>NLSDVDLSKYITTIAGVMTLSQVKGFVRKNGVNEAKIDEIKNDNVQDTAEQKVQLLRNWHQLHGKKEAYDTLIKDLKKANLCTLAEKIQTIILKDITSDSENSNFRNEIQSLVLE[8x];>[8x]GEEDLCAAFNVICDNVGKDWRRLARQLKVSDTKIDSIEDRYPRNLTERVRESLRIWKN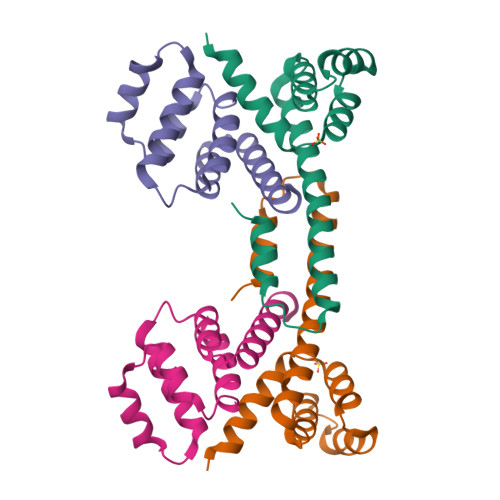TEKENATVAHLVGALRSCQMNLVADLVQEVQQARDLQNRSGAMSPMSWNSDASTSEASHHHHHH>AGLKLMGAPVKLTVSQGQPVKLNCSVEGMEEPDIQWVKDGAVVQNLDQLYIPVSEQHWIGFLSLKSVERSDAGRYWCQVEDGGETEISQPVWLTVEGVPFFTVEPKDLAVPPNAPFQLSCEAVGPPEPVTIVWWR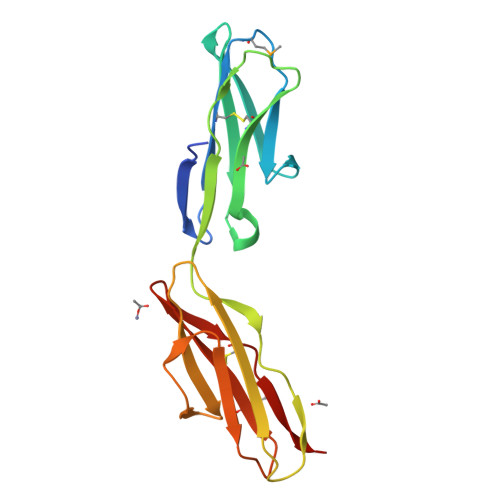GTTKIGGPAPSPSVLNVTGVTQSTMFSCEAHNLKGLASSRTATVHLQ[2x]[(2R)-1-(6-aminopurin-9-yl)propan-2-yl]oxymethyl-phosphonooxy-phosphinic acid | C9 H15 N5 O7 P2 | 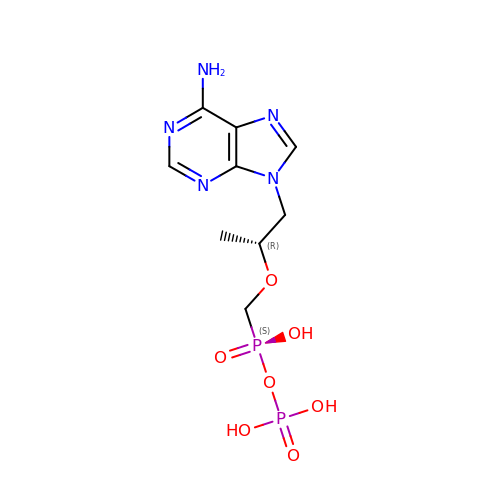BQDRSOMUPPCKPB-ZCFIWIBFSA-N>MNVDPFSPHSSDSFAQAASPARKPPRGGRRIWSGTREVIAYGMPASVWRDLYYWALKVSWPVFFASLAALFVVNNTLFALLYQLGDAPIANQSPPGFVGAFFFSVETLATVGYGDMHPQTVYAHAIATLEIFVGMSGIALSTGLVFARFARPRAKIMFARHAIVRPFNGRMTLMVRAANARQNVIAEARAKMRLMRREHSSEGYSLMKIHDLKLVRNEHPIFLLGWNMMHVIDESSPLFGETPESLAEGRAMLLVMIEGS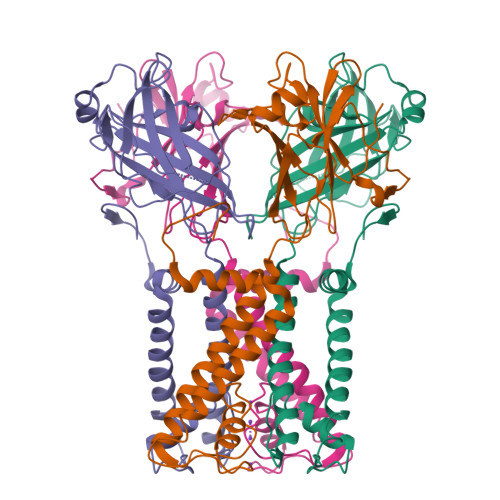DETTAQVMQARHAWEHDDIRWHHRYVDLMSDVDGMTHIDYTRFNDTEPVEPPGAAPDAQAFAAKPGEGDARPV[2x]>SNAMIKSWKPQELSISYHQFTVFQKDSTPPVMDWTDEAIEKGYAAADGAISFEAQRNTKAFILFRLNSSETVNSYEKKVTVPFHVTENGIHIESIMSKRLSFDLPKGDYQLTCWTVPAEMSDLHADTYIIDAV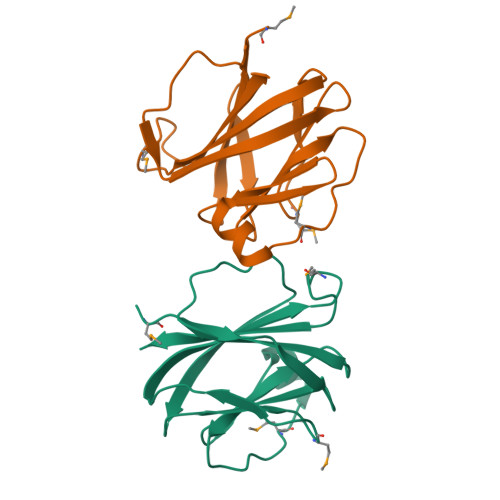SV[4x]>SELLVYMNGEFVPESQAKVSVFDHGFLYGDGVFEGIRAYNGKVFKLYEHIDRLYDCARVIDLKIPLSKEEFAEAILETLRRNNLRDAYIRPIVTRGAGDLGLDPRKCPSPNVIIITKPWGKLYGDLYEKGLKAITVAIRRNAIDSLPPNIKSLNYLNNILAKIEANAKGGDEAIFLDHNGYISEGSGDNIFIVKNGTITTPPTLNNLKGITRQVVIELINELEIPFREANIG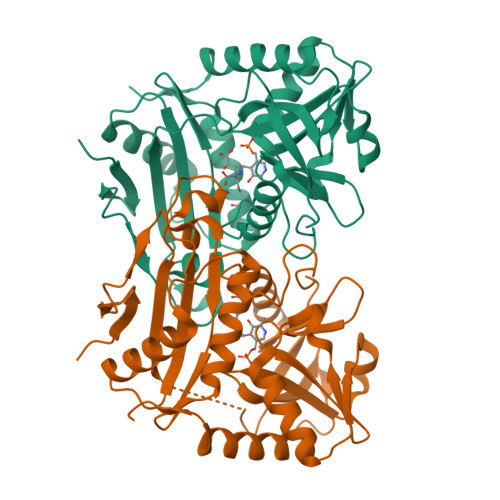LFDLYSADEIFVTGTAAEIAPVTYIDGRTVGNGKPGKVTKMLMEKFRERTENEGVEIYR[3x]>[10x]MNFGAFSINPAMMA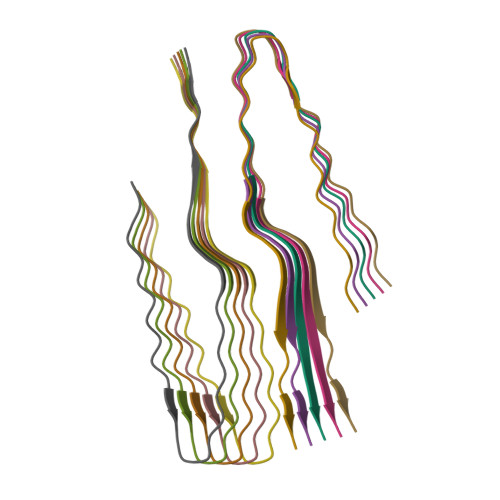AAQAALQSSWGMMGMLASQQNQSGPSGNNQNQGNMQ> GVPTYL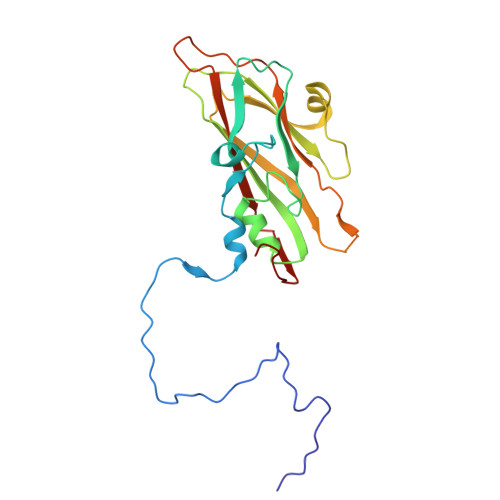LPGSSQFMTTDDHSSAPAFPDFSPTPEIHIPGRVHNMLELVQVESMMEINNVAGSSGMERLRVEISVQTDMDALLFNIPLDIQLDGPLRSTLLANIARYYTHWSGSMEMTFMFCGSFMATGKVILCYTPPGGSCPTDRESAMLGTHIVWDFGLQSSITLVIPWISGSHFRMFNSDAKSINANVGYVTCFMQTNLIVPKEAATSTYIIGFAAAKNDFSLRLMRDSPDI>[2x]SSITENTSWNKEFSAEAVNGVFVLCKSSSKSCATNNLARASKEYLPASTFKIPNAIIGLETGVIKNEHQVFK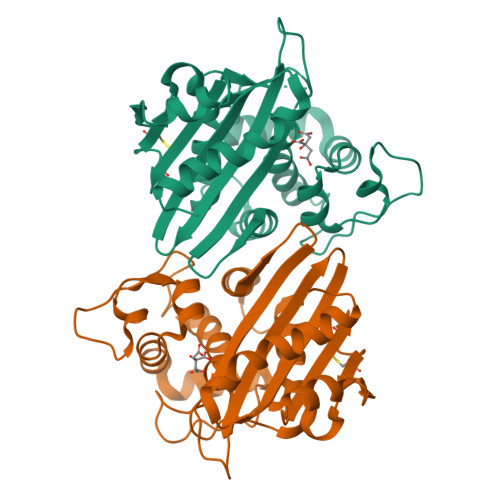WDGKPRAMKQWERDLSLRGAIQVSAVPVFQQIAREVGEVRMQKYLKKFSYGNQNISGGIDKFWEGQLRISAVNQVEFLESLFLNKLSASKENQLIVKEALVTEAAPEYLVHSKTGFSGVGTESNPGVAWWVGWVEKGTEVYFFAFNMDIDNENKLPLRKSIPTKIMASEGIIGG> SDAERDALNIETAIKTKGVDEVTIVNILTNRSNAQRQDIAFAYQRRTKKELASALKSALSGHLETVILGLLKTPAQYDASELKASMKGLGTDEDSLIEIICSRTNQELQE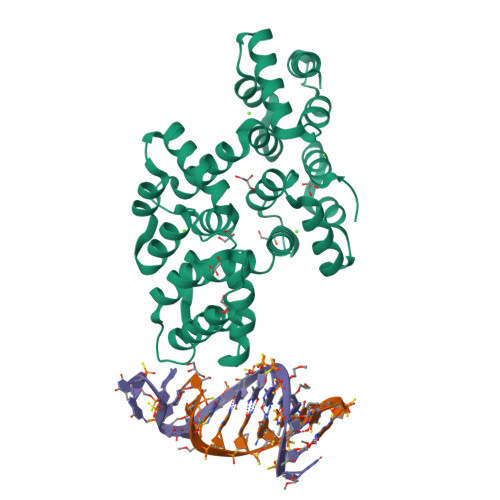INRVYKEMYKTDLEKDIISDTSGDFRKLMVALAKGRRAEDGSVIDYELIDQDARDLYDAGVKRKGTDVPKWISIMTERSVPHLQKVFDRYKSYSPYDMLESIRKEVKGDLENAFLNLVQCIQNKPLYFADRLYDSMKGKGTRDKVLIRIMASRSEVDMLKIRSEFKRKYGKSLYYYIQQDTKGDYQKALLYLCGGDD>[2x]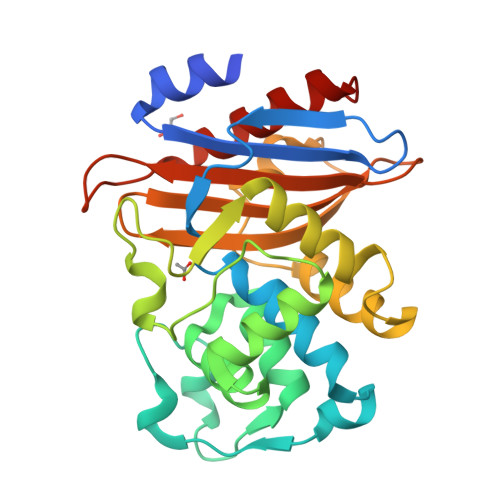GPMKTEMKDDFAKLEEQFDAKLGIFALDTGTNRTVAYRPDERFAFASTIKALTVGVLLQQKSIEDLNQRITYTRDDLVNYNPITEKHVDTGMTLKELADASLRYSDNAAQNLILKQIGGPESLKKELRKIGDEVTNPERFHPELNEVNPGETQDTSTARALVTSLRAFALEDKLPSEKRELLIDWMKRNTTGDALIRAGVPDGWEVADKTGAASYGTRNDIAIIWPPKGDPVVLAVLSSRDKKDAKYDDKLIAEATKVVMKALNMNGK> MEYEWKPDEQGLQQILQLLKESQSPDTTIQRTVQQKLEQLNQYPDFNNYLIFVLTKLKSEDEPTRSLSGLILKNNVKAHFQNFPNGVTDFIKSECLNNIGDSSPLIRATVGILITTIASKGELQNWPDLLPKLCSLLDSEDYNTCEGAFGALQKICEDSAEILDSDVLDRPLNIMIPKFLQFFKHSSPKIRSHAVACVNQFIISRTQALMLHIDSFIENLFALAGDEEPEVRKNVCRALVMLLEVRMDRLLPHMHNIVEYMLQRTQDQDENVALEACEFWLTLAEQPICKDVLVRHLPKLIPVLVNGMKYSDIDIILLKGDVEEDETIPDSEQDIRPRFHRSRTVAQQHDEDGIEEEDDDDDEIDDDDTISDWNLRKCSAAALDVLANVYRDELLPHILPLLKELLFHHEWVVKESGILVLGAIAEGCMQGMIPYLPELIPHLIQCLSDKKALVRSITCWTLSRYAHWVVSQPPDTYLKPLMTELLKRILDSNKRVQEAACSAFATLEEEACTELVPYLAYILDTLVFAFSKYQHKNLLILYDAIGTLADSVGHHLNKPEYIQMLMPPLIQKWNMLKDEDKDLFPLLECLSSVATALQSGFLPYCEPVYQRCVNLVQKTLAQAMLNNAQPDQYEAPDKDFMIVALDLLSGLAEGLGG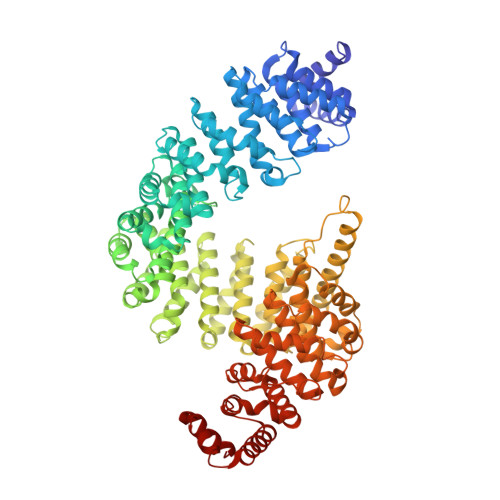NIEQLVARSNILTLMYQCMQDKMPEVRQSSFALLGDLTKACFQHVKPCIADFMPILGTNLNPEFISVCNNATWAIGEISIQMGIEMQPYIPMVLHQLVEIINRPNTPKTLLENTAITIGRLGYVCPQEVAPMLQQFIRPWCTSLRNIRDNEEKDSAFRGICTMISVNPSGVIQDFIFFCDAVASWINPKDDLRDMFCKILHGFKNQVGDENWRRFSDQFPLPLKERLAAFYGV>[12x]MKYVVVSGGVISGIGKGVLASSTGMLLKTLGLKVTSIKIDPYMNIDAGTMSPLEHGECFVLDDGGETDLDLGNYERYLGITLSRDHNITTGKIYSHVISRERRGDYLGKTVQIVPHLTNAIQDWIQRVSKIPVDDTGLEPDVCIIELGGTVGDIESAPFVEALRQFQFEVGRENFALIHVSLVPVIHGEQKTKPTQAAIKDLRSLGLIPDMIACRCSEELNRSTIDKIAMFCHVGPEQVVNVHDVNSTYHVPLLLLKQHMIDYLHSRLKLGEVPLTLEDKERGSQLLTNWENMTKNLDDSDDVVKIALVGKYTNLKDSYLSVTKSLEHASMKCRRQLEILWVEASNLEPETQEVDKNKFHDSWNKLSSADGILVPGGFGTRGIEGMILAAKWARESGVPFLGVCLGLQVAAIEFARNVIGRPNSSSTEFLDETLLAPEDQVVITMRLGLRPTIFQPNSEWSNIRKLYGEVNEVHERHRHRYEINPKIVNDMESRGFIFVGKDETGQRCEIFELKGHPYYVGTQYHPEYTSKVLEPSRPFWGLVAAASGTLGEVIKDINL

CTP synthase (CTPS) catalyzes the final, rate-limiting step of de novo CTP biosynthesis (Lieberman, 1956). Each CTPS monomer consists of a glutaminase domain and an amido-ligase domain connected by an alpha helical linker. Glutamine hydrolysis in the glutaminase domain produces ammonia which is transferred through a channel into the amido-ligase domain, where it is ligated to UTP to form CTP in an ATP-dependent process. Budding yeast have two CTPS isoforms, Ura7 and Ura8, which share 78 % identical residues.

To enable structure determination, we assembled filaments at pH 6.5, where single filaments predominate over larger bundles. We solved filament structures of both Ura7 and Ura8 in substrate- (ATP and UTP) and product- (CTP) bound states. Ura8 yielded the highest resolution structures, at 2.8 Å (substrates) and 3.8 Å (products). In the Ura8 structures, all ligands were clearly visible and bound as previously described for other CTPS homologs, including an imino-phosphate reaction intermediate recently observed in Drosophila CTPS, and the presence of two distinct CTP-binding sites per monomer recently reported in human and Drosophila CTPS (Endrizzi et al., 2004; Goto et al., 2004; Lynch et al., 2021; Lynch et al., 2017; Lynch and Kollman, 2020; Zhou et al., 2021). Helix 356–370 in the glutaminase domain mediates interactions between tetramers, so that each protomer is involved in assembly contacts. His360 interacts with D370 which would be stabilized by protonation of His360 at low pH, and likely explains the pH-sensitivity of the assembly interaction. We see density consistent with two rotamer positions of H360 that may reflect partial protonation of the sidechain at pH 6.5. One rotamer that likely reflects the protonated state interacts with D370, and the other rotamer that likely reflects an unprotonated state forms a hydrogen bond to a backbone carbonyl across the interface. The Ura8 product-bound filament is in the canonical inhibited conformation, but the substrate-bound structure is in a conformation intermediate between canonical active and inhibited states, in which the ammonia channel remains closed. This suggested to us that one function of yeast CTPS filaments is to constrain the enzyme in a low activity conformation.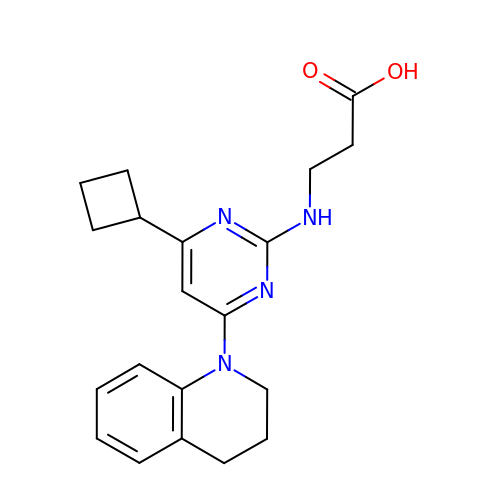3-[[4-cyclobutyl-6-(3,4-dihydro-2~{H}-quinolin-1-yl)pyrimidin-2-yl]amino]propanoic acid | C20 H24 N4 O2 | PUOUMWUWJBCLCR-UHFFFAOYSA-N>[2x]MTKNKMEAKIDELINNDPVWSSQNESLISKPYNHILLKPGKNFRLNLIVQINRVMNLPKDQLAIVSQIVELLHNSSLLIDDIEDNAPLRRGQTTSHLIFGVPSTINTANYMYFRAMQLVSQLTTKEPLYHNLITIFNEELINLHRGQGLDIYWRDFLPEIIPTQEMYLNMVMNKTGGLFRLTLRLMEALSPSSHHGHSLVPFINLLGIIYQIRDDYLNLKDFQMSSE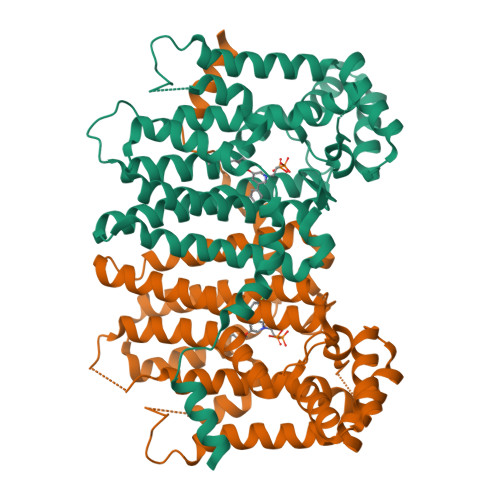KGFAEDITEGKLSFPIVHALNFTKTKGQTEQHNEILRILLLRTSDKDIKLKLIQILEFDTNSLAYTKNFINQLVNMIKNDNENKYLPDLASHSDTATNLHDELLYIIDHLSEL>EFQVLFVLTILTLISGTIFYSTVEGLRPIDALYFSVVTLTTVGYGDFSPQTDFGKIFTILYIFIGIGLVFGFIHKLAVNVQLPSILSNL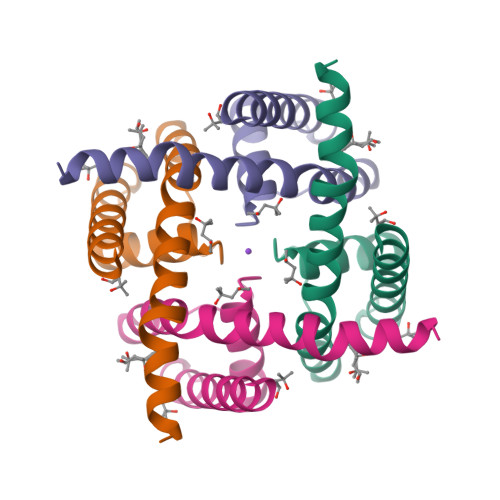VPR[2x]3-(3-carbamimidoylphenyl)-N-(2'-sulfamoylbiphenyl-4-yl)-1,2-oxazole-4-carboxamide | 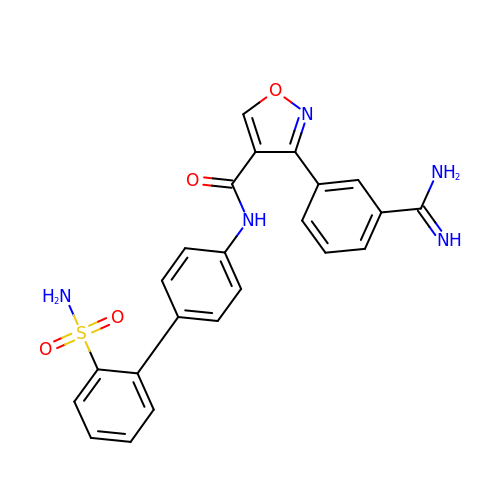C23 H19 N5 O4 S | LPYBKEFBMJIVEB-UHFFFAOYSA-N> DEDREWIERFNRILIESLTTGDEHTLKELIDPNARLVINGRDIHGREEFVRLLSEMGVKHFHVHDVKVVGNKAVTRGILYFN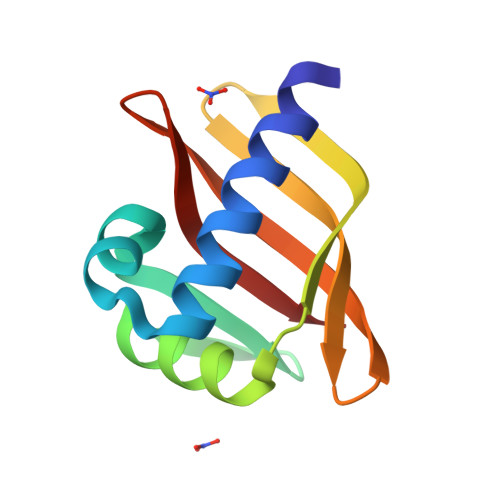GREYDVDVFTRKIDGRWLYESLEVK4-[3-[3-[2,4-bis(azanyl)-6-ethyl-pyrimidin-5-yl]prop-2-ynyl]-5-methoxy-phenyl]benzoic acid | C23 H22 N4 O3 | 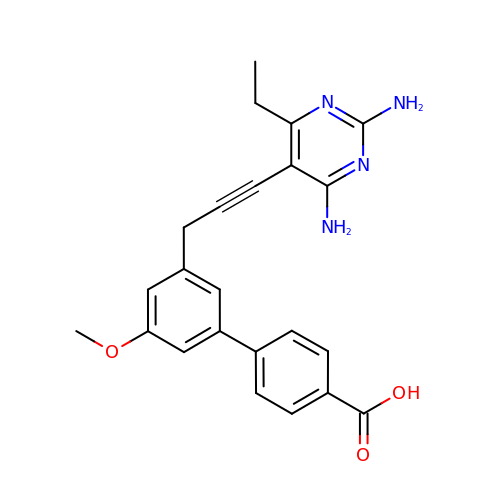VLQRVOAJCWFFQG-UHFFFAOYSA-N>[4x]MGHHHHHHMYTDLKDKVVVITGGSTGLGRAMAVRFGQEEAKVVINYYNNEEEALDAKKE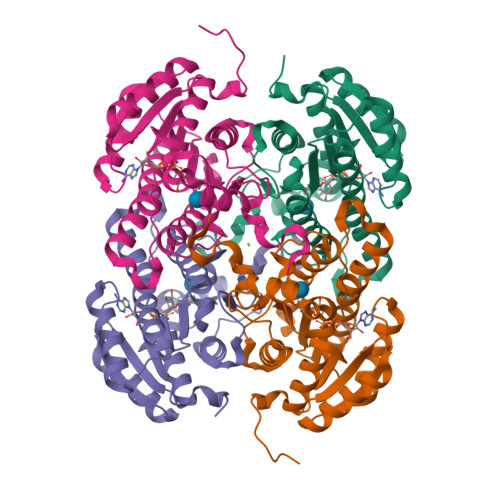VEEAGGQAIIVQGDVTKEEDVVNLVQTAIKEFGTLDVMINNAGVENPVPSHELSLDNWNKVIDTNLTGAFLGSREAIKYFVENDIKGNVINMSSVHEMIPWPLFVHYAASKGGMKLMTETLALEYAPKGIRVNNIGPGAMNTPINAEKFADPVQRADVESMIPMGYIGKPEEVAAVAAFLASSQASYVTGITLFADGGMTKYPSFQFGRG> MKHHHHHHPEIEKAQREIIEAFNAKPKNGINKIKEICEQYKISPNEEIAEFFHQQRKNLDLEAVGDYLSSPEAENQQVLKAFTSQMNFNGQSFVEGLRTFLKTFKLPGEAQKIDRLVQSFSGAYFQQNPDVVSNADAAYLLAFQTIMLNTDLHNPSIPEKNKMTVYGLKRNLRGGNNGGDFDAKFLEELYSEIKAKPFELNFVDSSPGYQINNISSQNDKTFKQLNQFLEEKRNIQNIFPKLQNNNLTIEFKNPKTFLSKFTGYKGSVIIKDEKSGAAEIQVYKPSIFSRWFLGEKSKIIIQPLREEGRQPSEQSLKLA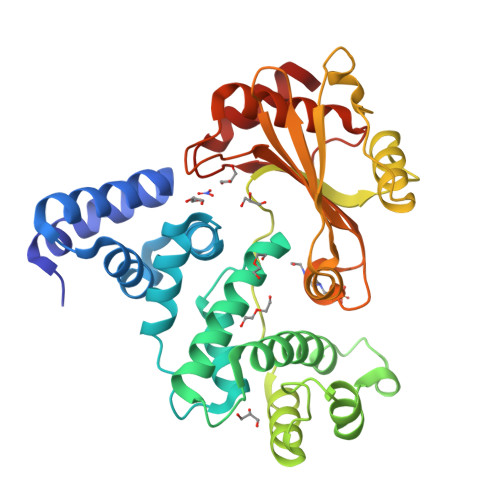AQITASFETKVTSIKATYDYLKEDLKSQYDNIR> GESQEDMFAKLK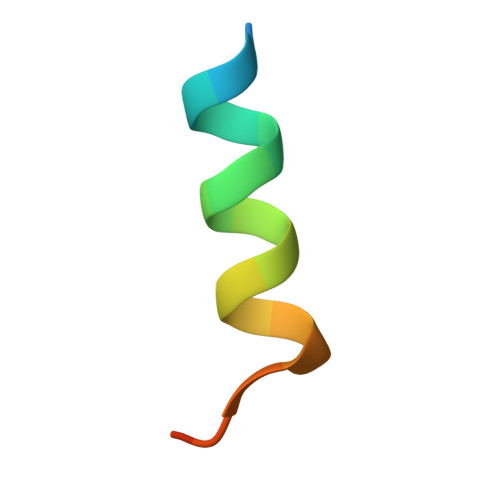DKFFNEINK> SS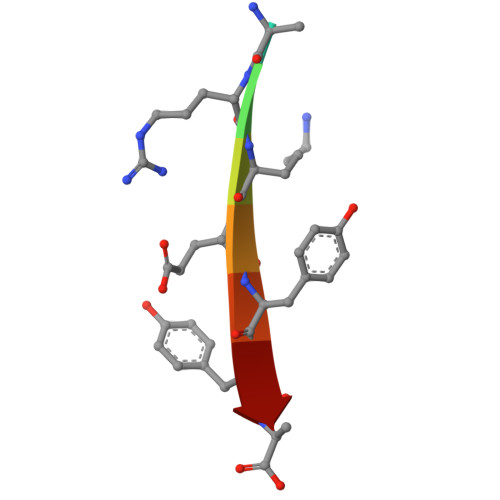RKEYYA>[2x]MQPASAKWYDRRDYVFIEFCVEDSKDVNVNFEKS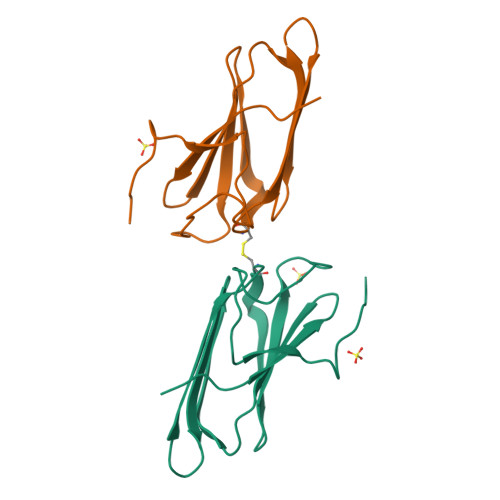KLTFSCLGGSDNFKHLNEIDLFHCIDPNDSKHKRTDRSILCCLRKGESGQSWPRLTKERAKLNWLSVDFNNWKDWEDDSDEDMSNFDRFSE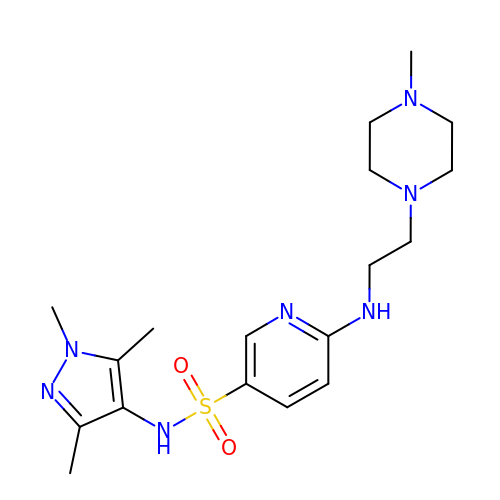6-{[2-(4-METHYLPIPERAZIN-1-YL)ETHYL]AMINO}-N-(1,3,5-TRIMETHYL-1H-PYRAZOL-4-YL)PYRIDINE-3-SULFONAMIDE | C18 H29 N7 O2 S | RLKMGPCSKXTKNK-UHFFFAOYSA-N> MGWSCIILFLVATATGVHSNPPTFSPALLVVTEGDSATFTCSFSSTSESFVLNWYRMSPSGQPDKLAAFPEDRSQPGQDSRFRVTQLPNGRDFHMSVVRARRDDSGTYLCGAISLAPKVQIKESLRAELRVTERRAEPEA;> MIFLLLMLSLELQLHQIAALFTVTVPKELYIIEHGSDVTLECNFDTGSHVNLGAITASLQKVEDDTSPHRERATLLEEQLPLGKASFHIPQVQVR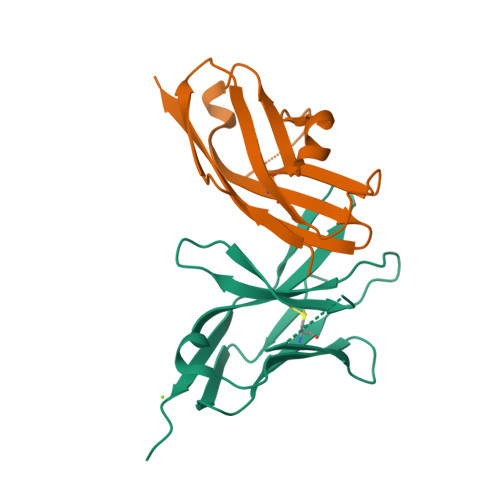DEGQYQCIIIYGVAWDYKYLTLKVKASY>AYSNTYQEFTNIDQAKAWGNAQYKKYGLSKSEKEAIVSYTKSASEINGKLRQNKGVINGFPSNLIKQVELLDKSFNKMKTPENIMLFRGDDPAYLGTEFQNTLLNSNGTINKTAFEKAKAKFLNKDRLEYGYISTSLMNVSQFAGRPIITKFKVAK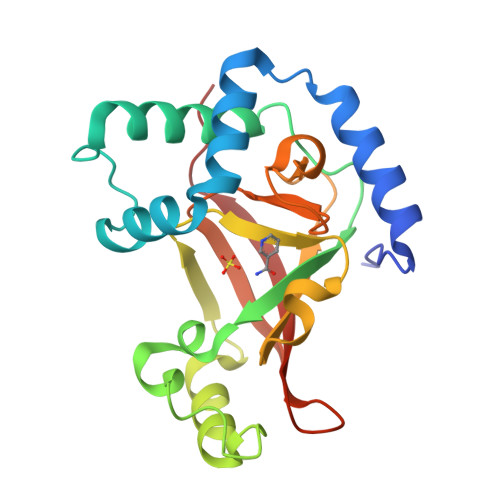GSKAGYIDPISAFAGQLEMLLPRHSTYHIDDMRLSSDGKQIIITATMMGTAINPK[4x]> AEEWYFGKITRRESERLLLNPENPRGTFLVRESET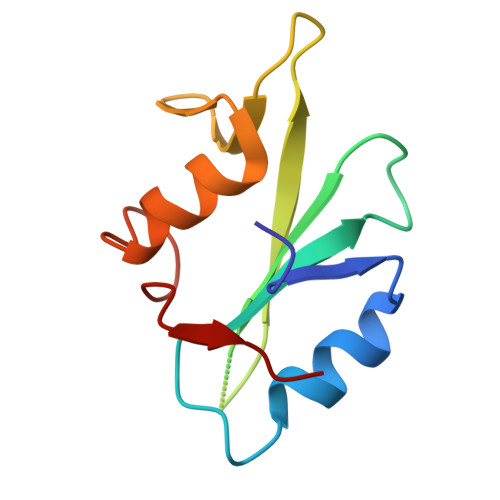TKGAYCLSVSAFANAKGLNVAHYKIRKLDSGGFYITSRTQFSSLQQLVAYYSKHADGLCHRLTNVCPT> GSHMEAVQNRIVEAAERVPGVRGVIHLRARYVGQDIWADMIIGVDPENTVEQAAEICEAVQAAVCGKIRRIESLHVSAEAREIGDTTKPSFSDQPLSFDEVMLSKVDN

One group of metal ion efflux transporters that regulates metal ion homeostasis and can be found in all domains of life is the Cation Diffusion Facilitator (CDF) protein family. One of the most highly conserved and abundant integral MM proteins is the CDF transporter MamM. MamM was recently proposed to function as a magnetosome-directed iron transporter required for iron biomineralization since its deletion abolished magnetite biomineralization and mutation of residues within the conserved TMD metal-binding site resulted in alterations of magnetite crystal size, morphology and even mineral phase. To summarize our results we present an alternative model for the CDF CTD mode of action, in which we propose that upon metal cation binding, the CTD induces conformational changes towards a tighter and more compact fold which allows the activation of iron transport through the TMD.

Examining this closed state model, three putative binding sites were revealed, in which Asp, Glu and His residues from the two monomers are brought into close proximity and may bind divalent cations. The central binding site is presumed to be the main site as it displays tight packing and contains two symmetry-related His285 and two Asp249 residues. The other two symmetrical peripheral binding sites contain His264 and Glu289 residues but no designated binding cavity was found. Compared to transcomplementation with the wild-type allele, single point mutations of the histidine residues at the putative central binding site (H285A) or periphery binding sites (H264A) affected neither Cmag values nor the number, size and morphology of the crystals. The D249A, H285A and H264A mutants displayed a minor increase in the number of binding sites compared to the wild-type protein, which may be the result of an increased void volume that allowed the accommodation of additional cations after amino acid substitution to alanine. Since Glu289 is located at the domain surface, it is more likely to have a role in peripheral binding site stabilization and metal ion coordination than the relatively buried His264. Fourth, we confirmed metal coordination by the His264 and His285 residues by ssNMR. To confirm that these observed phenotypic differences are due to true transport function alternations, we also examined the expression levels of all MamM mutants, their ability to stabilize MamB expression, performed MD simulations for dimer stability evaluation and determined their CTD structures. (ii) All mutants exhibited an apo-MamM CTD-like behavior along the MD simulations (see Fig. B in file S1 for representative MD simulations), and (iii) an absence of structural differences was observed.>MRGSHHHHHHGSACELSECPVRKSNVGGGGTRNHD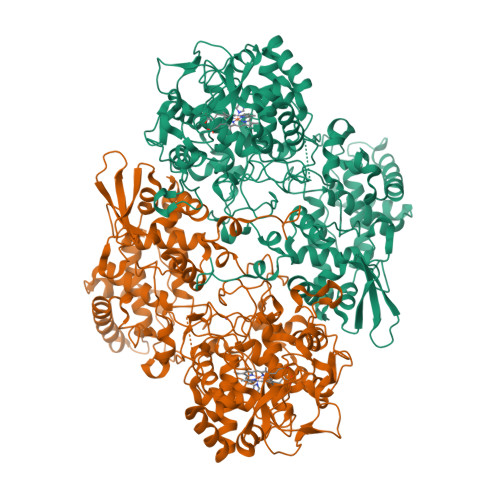WWPAQLRLNILRQHTPVSNPLDKDFDYAAAFKSLDYEGLKKDLTKLMTDSQDWWPADFGHYGGLFIRMAWHSAGTYRVTDGRGGGGEGQQRFAPLNSWPDNVSLDKARRLLWPIKQKYGNKISWSDLLLLTGNVALESMGFKTFGFAGGRPDTWEADESVYWGAETTWLGNEDRYSEGQEGHEGHGVVQGDESKKQHTDIHNRDLQSPLASSHMGLIYVNPEGPDGIPDPVASAKDIRVTFGRMAMNDEETVALIAGGHSFGKTHGAGPTHHVGKEPEAAPIEHQGLGWANSFGQGKGPDTITSGLEVTWTPTPTKWGMGYLEYLYKFDWEPTKSPAGANQWVAKNAEPTIPDAYDPNKKKLPTMLTTDIALRMDPAYDKICRDYLANPDKFADAFARAWFKLLHRDMGPRTRWIGPEVPSEILPWEDYIPPVDYQIIDDNDIAALKKEILATGVAPKKLIFVAWSSASSFRGSDKRGGANGARIRLAPQNEWKVNDPSTLREVLAALESVQQKFNDSSSGKKVSLADLIVLGGVAALEQASGLVVPFTPGRNDATQEHTDVHSFTHLEPHADGFRSYGKGTKRVRTEQFLIDRASLLTLSAPELTALIGGLRVLEANYDGSSYGVLTKTPGKLTNDYFVNLLDTNTAWKAADNEGEVFIGYDRKTHDKKWTATRADLIFGAHAELRALAEVYAAVDGEEKFKRDFVAAWHKVMNLDRFDLKQEGRGQNAPKL[2x]> IVNPLFQ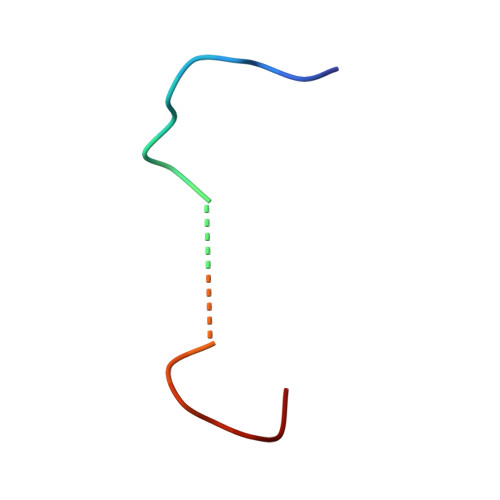LGLQREVNNDSFNEFDSQT>[8x]MTQPMPGKPAEDAENELDIRGLFRTLWAGKLWI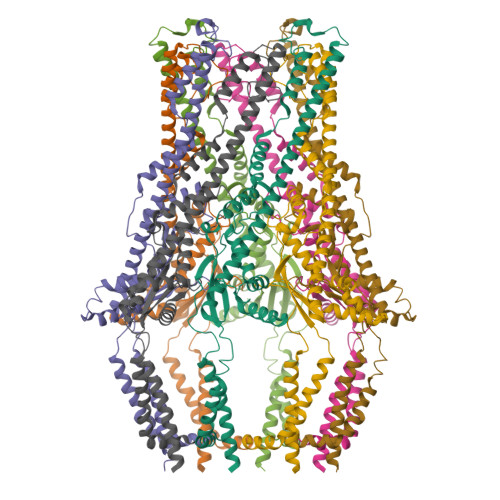IGMGLAFALIALAYTFFARQEWSSTAITDRPTVNMLGGYYSQQQFLRNLDVRSNMASADQPSVMDEAYKEFVMQLASWDTRREFWLQTDYYKQRMVGNSKADAALLDEMINNIQFIPGDFTRAVNDSVKLIAETAPDANNLLRQYVAFASQRAASHLNDELKGAWAARTIQMKAQVKRQEEVAKAIYDRRMNSIEQALKIAEQHNISRSATDVPAEELPDSEMFLLGRPMLQARLENLQAVGPAFDLDYDQNRAMLNTLNVGPTLDPRFQTYRYLRTPEEPVKRDSPRRAFLMIMWGIVGGLIGAGVALTRRCSKEFRVPGSHHHHHHHH>GACGCCGGUGGUGGCACUCCUGGUUUUCAGGACGGGGUUCAAUUCCCUGCGGUGUC[2x]

The AS and TSL stack to form one continuous helical stack containing four GU base pairs, while the AC and DSL form another. The two helices are held in a roughly perpendicular orientation by interactions between the elements that are analogous to the D and T loops in tRNA.

We have determined the crystal structures of human mascRNA at 2.40 Å, human menRNA at 2.23 Å, and medaka mascRNA at 2.28 Å. The structure of medaka mascRNA at 2.28 Å was solved using the single-wavelength anomalous dispersion method, while the remaining structures were solved by molecular replacement, using the former as a reference model. We further conducted a cross-species comparison of mascRNA between humans and medaka. Despite fewer GU base pairs in the AS and a more compact D loop due to the lack of a uracil nucleotide in medaka mascRNA, both structures superimpose well with each other with an RMSD of 2.2 Å. In medaka mascRNA, the base triple is formed by a hydrogen bond donated from the N4 of C15 to the O4 of U43, coupled with the G10–C15 base pair of D stem, which is comparable to the C16–G10–A44 triple in human mascRNA. Furthermore, the hydrogen bond donated from G11 N1 to U44 C6 is analogous to the interaction between U12 N3 and U45 O2 in human mascRNA. The high degree of structural similarity observed in mascRNAs between medaka and humans implies a strong selective pressure to maintain these elements.>[2x]MGLMNAFDSQTEDSSPAIGRNLRSRPLARKKLSEMVEEELEQMIRRREFGEGEQLPSERELMAFFNVGRPSVREALAALKRKGLVQINNGERARVSRPSADTIIGELSGMAKDFLSHPGGIAHFEQLRLFFESSLVRYAAEHATDEQIDLLAKALEINSQSLDNNAAFIRSDVDFHRVLAEIPGNPIFMAIHVALLDWLIAARPTVTDQALHEHNNVSYQQHIAIVDAIRRHDPDEADRALQSHLNSVSATWHAFGQTTNKKK

The Escherichia coli GntR-type transcriptional repressor, NanR, regulates sialic acid metabolism, but the mechanism is unclear. Analogous to other GntR members, the NanR monomer has a two-domain architecture, comprising an N-terminal winged helix–turn–helix DNA-binding domain (α1–α3, β1–β2, green) linked to an α-helical C-terminal effector-binding domain (α4–α10, tan). Here, we demonstrate that three NanR dimers bind a (GGTATA)3-repeat operator cooperatively and with high affinity. The effector, N-acetylneuraminate, binds NanR and attenuates the NanR-DNA interaction.

We used the (GGTATA)2-repeat oligonucleotide to solve this structure as NanR bound poorly to the oligonucleotide with only one GGTATA repeat. NanR binds DNA in an asymmetric pose relative to the DNA helix. The C-terminal domain closely matched that found in the NanR crystal structure (RMSD = 2.1 Å), showing that DNA binding does not markedly alter C-terminal domain architecture. However, the direction, length, and position of the α4-linking helices are altered when compared to the crystal structure. In contrast, when bound to DNA in the cryo-EM structure, we observed that the α4-linking helices are oriented in a different direction and adopt a more extended conformation (green and black). The α2- and α3-helices of each N-terminal DNA-binding domain make contact at the major groove, whereas the α1-helices interact with the DNA phosphate backbone. Comparatively, monomer A is better resolved, particularly in the wing motif and the α3-helix, which allowed several of the putative DNA-binding sidechains, such as Arg73, to be assigned in the model. Despite the assignment of these putative DNA-binding residues based on these inferences, it is important to note that the resolution of the overall DNA-binding region (~5 Å) is insufficient to resolve specific DNA base pair contacts with the (GGTATA)2-repeat oligonucleotide. However, unlike FadR, where each N-terminal domain binds a palindromic DNA sequence symmetrically, NanR binds a repeat sequence with one N-terminal domain of the dimer engaging the consensus (GGTATA) sequence and the other N-terminal domain binding an adjacent non-consensus DNA sequence.> QSVEESEGGLFKPTDTLTLTCTA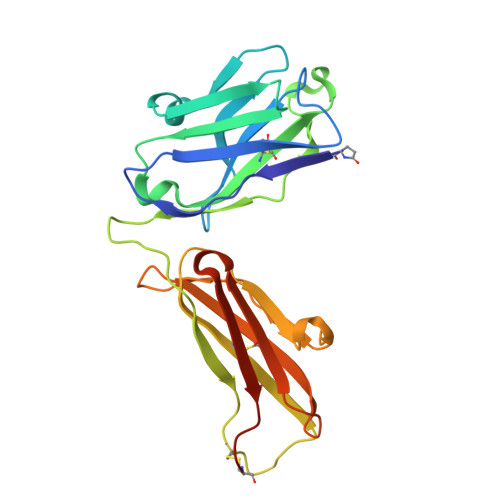SGFSLSGHGVIWVRQAPGKGLEWIGSAGAYGRIYYASWAKSRSTITRNTNLNTVTLKMTSLTAADTATYFCARRSDVGTSVGFDSWGPGTLVTISSSSGQPKAPSVFPLAPCCGDTPSSTVTLGCLVKGYLPEPVTVTWNSGTLTNGVRTFPSVRQSSGLYSLSSVVSVTSSSQPVTCNVAHPATNTKVDKTVAPSTCSHHHHHH> MEPHVLGAGLYWLLLPCTLLAASLLRFNALSLVYLLFLLLLPWLPGPSRHSIPGHTGRLLRALLCLSLLFLVAHLAFQICLHTVPHLDQFLGQNGSLWVKVSQHIGVTRLDLKDIFNTTRLVAPDLGVLLASSLCLGLCGRLTRKAGQSRRTQELQDDDDDDDDDDEDIDAAPAVGLKGAPALATKRRLWLASRFRVTAHWLLMTSGRTLVIVLLALAGIAHPSAFSSIYLVVFLAICTWWSCHFPLSPLGFNTLCVMVSCFGAGHLICLYCYQTPFIQDMLPPGNIWARLFGLKNFVDLPNYSSPNALVLNTKHAWPIYVSPGILLLLYYTATSLLKLHKSCPSELRKETPREDEEHELELDHLEPEPQARDATQGEMPMTTEPDLDNCTVHVLTSQSPVRQRPVRPRLAELKEMSPLHGLGHLIMDQSYVCALIAMMVWSIMYHSWLTFVLLLWACLIWTVRSRHQLAMLCSPCILLYGLTLCCLRYVWAMELPELPTTLGPVSLHQLGLEHTRYPCLDLGAMLLYLLTFWLLLRQFVKEKLLKKQKVPAALLEVTVADTEPTQTQTLLRSLGELVTGIYVKYWIYVCAGMFIVVSFAGRLVVYKIVYMFLFLLCLTLFQVYYTLWRKLLRVFWWLVVAYTMLVLIAVYTFQFQDFPTYWRNLTGFTDEQLGDLGLEQFSVSELFSSILIPGFFLLACILQLHYFHRPFMQLTDLEHVPPPGTRHPRWAHRQDAVSEAPLLEHQEEEEVFREDGQSMDGPHQATQVPEGTASKWGLVADRLLDLAASFSAVLTRIQVFVRRLLELHVFKLVALYTVWVALKEVSVMNLLLVVLWAFALPYPRFRPMASCLSTVWTCIIIVCKMLYQLKIVNPHEYSSNCTEPFPNNTNLQPLEINQSLLYRGPVDPANWFGVRKGYPNLGYIQNHLQILLLLVFEAVVYRRQEHYRRQHQQAPLPAQAVCADGTRQRLDQDLLSCLKYFINFFFYKFGLEICFLMAVNVIGQRMNFMVILHGCWLVAILTRRRREAIARLWPNYCLFLTLFLLYQYLLCLGMPPALCIDYPWRWSKAIPMNSALIKWLYLPDFFRAPNSTNLISDFLLLLCASQQWQVFSAERTEEWQRMAGINTDHLEPLRGEPNPIPNFIHCRSYLDMLKVAVFRYLFWLVLVVVFVAGATRISIFGLGYLLACFYLLLFGTTLLQKDTRAQLVLWDCLILYNVTVIISKNMLSLLSCVFVEQMQSNFCWVIQLFSLVCTVKGYYDPKEMMTRDRDCLLPVEEAGIIWDSICFFFL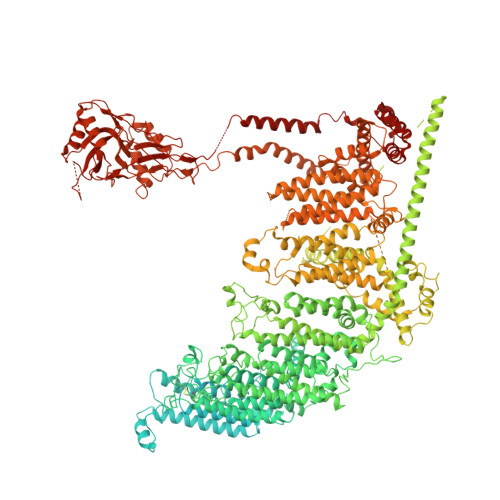LLQRRIFLSHYFLHVSADLKATALQASRGFALYNAANLKSINFHRQIEEKSLAQLKRQMKRIRAKQEKYRQSQASRGQLQSKDPQDPSQEPGPDSPGGSSPPRRQWWRPWLDHATVIHSGDYFLFESDSEEEEEALPEDPRPAAQSAFQMAYQAWVTNAQTVLRQRRERARQERAEQLASGGDLNPDVEPVDVPEDEMAGRSHMMQRVLSTMQFLWVLGQATVDGLTRWLRAFTKHHRTMSDVLCAERYLLTQELLRVGEVRRGVLDQLYVGEDEATLSGPVETRDGPSTASSGLGAEEPLSSMTDDTSSPLSTGYNTRSGSEEIVTDAGDLQAGTSLHGSQELLANARTRMRTASELLLDRRLHIPELEEAERFEAQQGRTLRLLRAGYQCVAAHSELLCYFIIILNHMVTASAASLVLPVLVFLWAMLTIPRPSKRFWMTAIVFTEVMVVTKYLFQFGFFPWNSYVVLRRYENKPYFPPRILGLEKTDSYIKYDLVQLMALFFHRSQLLCYGLWDHEEDRYPKDHCRSSVKDREAKEEPEAKLESQSETGTGHPKEPVLAGTPRDHIQGKGSIRSKDVIQDPPEDLKPRHTRHISIRFRRRKETPGPKGTAVMETEHEEGEGKETTERKRPRHTQEKSKFRERMKAAGRRLQSFCVSLAQSFYQPLQRFFHDILHTKYRAATDVYALMFLADIVDIIIIIFGFWAFGKHSAATDIASSLSDDQVPQAFLFMLLVQFGTMVIDRALYLRKTVLGKLAFQVVLVVAIHIWMFFILPAVTERMFSQNAVAQLWYFVKCIYFALSAYQIRCGYPTRILGNFLTKKYNHLNLFLFQGFRLVPFLVELRAVMDWVWTDTTLSLSNWMCVEDIYANIFIIKCSRETEKKYPQPKGQKKKKIVKYGMGGLIILFLIAIIWFPLLFMSLIRSVVGVVNQPIDVTVTLKLGGYEPLFTMSAQQPSIVPFTPQAYEELSQQFDPYPLAMQFISQYSPEDIVTAQIEGSSGALWRISPPSRAQMKQELYNGTADITLRFTWNFQRDLAKGGTVEYTNEKHTLELAPNSTARRQLAQLLEGRPDQSVVIPHLFPKYIRAPNGPEANPVKQLQPDEEEDYLGVRIQLRREQVGTGASGEQAGTKASDFLEWWVIELQDCKADCNLLPMVIFSDKVSPPSLGFLAGYGIVGLYVSIVLVVGKFVRGFFSEISHSIMFEELPCVDRILKLCQDIFLVRETRELELEEELYAKLIFLYRSPETMIKWTRERE>[8x]MGHPEEVDVIVCGGGPAGCVVAGRLAYADPTLKVMLIEGGANNRDDPWVYRPGIYVRNMQRNGINDKATFYTDTMASSYLRGRRSIVPCANILGGGSSINFQMYTRASASDWDDFKTEGWTCKDLLPLMKRLENYQKPCNNDTHGYDGPIAISNGGQIMPVAQDFLRAAH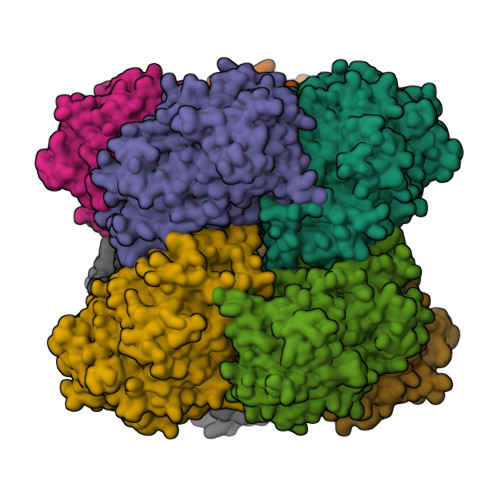AIGVPYSDDIQDLTTAHGAEIWAKYINRHTGRRSDAATAYVHSVMDVQDNLFLRCNARVSRVLFDDNNKAVGVAYVPSRNRTHGGKLHETIVKARKMVVLSSGTLGTPQILERSGVGNGELLRQLGIKIVSDLPGVGEQYQDHYTTLSIYRVSNESITTDDFLRGVKDVQRELFTEWEVSPEKARLSSNAIDAGFKIRPTEEELKEMGPEFNELWNRYFKDKPDKPVMFGSIVAGAYADHTLLPPGKYITMFQYLEYPASRGKIHIKSQNPYVEPFFDSGFMNNKADFAPIRWSYKKTREVARRMDAFRGELTSHHPRFHPASPAACKDIDIETAKQIYPDGLTVGIHMGSWHQPSEPYKHDKVIEDIPYTEEDDKAIDDWVADHVETTWHSLGTCAMKPREQGGVVDKRLNVYGTQNLKCVDLSICPDNLGTNTYSSALLVGEKGADLIAEELGLKIKTPHAPVPHAPVPTGRPATQQVR The African swine fever virus (ASFV) type II topoisomerase (Topo II), pP1192R, is the only known Topo II expressed by mammalian viruses and is essential for ASFV replication in the host cytoplasm. In ASFV, a functional viral Topo II pP1192R has been identified, encoded by a viral gene conserved in ASFV strains, P1192R. pP1192R is detectable at an intermediate to late stage of ASFV infection, mainly within the cytoplasmic virus factory, and has been confirmed to be important for ASFV replication. Topo IIAs exhibit a 2-fold symmetry and comprise two functional domains: an ATPase domain and a DNA binding/cleavage domain. The mechanism of enzymatic action involves the opening and closing of three gate-like dimeric interfaces, which are called the N-, DNA- and C-gate, respectively, upon ATP binding and hydrolysis and DNA cleavage that introduces a double-strand break in the DNA (G-segment) trapped in the DNA-gate for transport of another DNA strand (T-segment).

To provide detailed information of the ATPase domain and support the model building of the full-length pP1192R, the atomic resolution structure of the ATPase domain of pP1192R in complex with the nonhydrolyzable homolog of ATP (AMP-PNP) was determined by X-ray crystallography at 1.8 Å using a truncated pP1192R-ATPase protein expressed as soluble protein in E. coli cells. The electron density map is of good quality, with only a few flexible terminal residues and two regions containing R70-T76 and I334-R343 being disordered. Interestingly, the region R70-T76 was found to exhibit large conformational changes under different redox conditions, as detailed by Chang et al., involving the formation and breakage of the disulfide bond between C72 and C138, which may reflect a redox regulatory mechanism of pP1192R. Our structure shows high overall similarity to both the reduced and oxidized forms, with the RMSD values of 0.18 and 0.102 Å, respectively. The observed flexibility in this region of our structure may reflect an intermediate state that transitions to the reduced or oxidized conformation. The pP1192R-ATPase displayed a conserved heart-shaped dimeric architecture as its homologs with each protomer consisting of two well characterized regions, i.e. the N-terminal GHKL ATP-binding fold and the C-terminal Transducer domain. The bound AMP-PNP in the pP1192R ATPase adopts an identical orientation to that of the other Topo IIAs ATPases, and the secondary structure elements comprising the binding pocket are conserved. The primary interactions were correspondingly mediated by residues on the β4 strand, the α4 helix and the extended loop between the α5 and α6 helices, termed as the ‘ATP-lid’, with the previously defined QTK-loop of the transducer domain forming salt bridges with the γ-phosphate of AMP-PNP.

> METFEISDFKEHAKKKSMWAGALNKVTISGLMGVFTEDEDLMALPIHRDHCPALLKIFDELIVNATDHERACHNKTKKVTYIKISFDKGVFSCENDGPGIPIVKHEQASLIAKRDVYVPEVASCYFLAGTNINKAKDCIKGGTNGVGLKLAMVHSQWAILTTADGSQKYVQHINQRLDNIEPPTITPSREMFTRIELMPVYQELGYAQPLSETEQADLSAWIYLRACQCAAYVGKGTTIYYNDKPCSTSSVMALAKMYTLVTAPNSTIYTATIKADAKPYSLHPLQVAAVVSPKFKKFEHVSIINGVNCVKGEHVTFLKKAINEMVVKKFQQTIKDKNRKTTLRDSCSNIFVVIVGSIPGIEWTGQRKDELSIAENVFKTHYSIPSSFLTSMTRSIVDILLQS>GPEKIRPECFELLRVLGKGGYGKVFQVRKVTGANTGKIFAMKVLKKAMIVRNAKDTAHTKAERNILEEVKHPFIVDLIYAFQTGGKLYLILEYLSGGELFMQLEREGIFMEDTACFYLAEISMALGHLHQKGIIYRDLKPENIMLNHQGHVKLTDFGLCKESIHDGTVTHTFCGTIEYMAPEILMRSGHNRAVDWWSLGALMYDMLTGAPPFTGENRKKTIDKILKCKLNLPPYLTQEARDLLKKLLKRNAASRLGAGPGDAGEVQAHPFFRHINWEELLARKVEPPFKPLLQSEEDV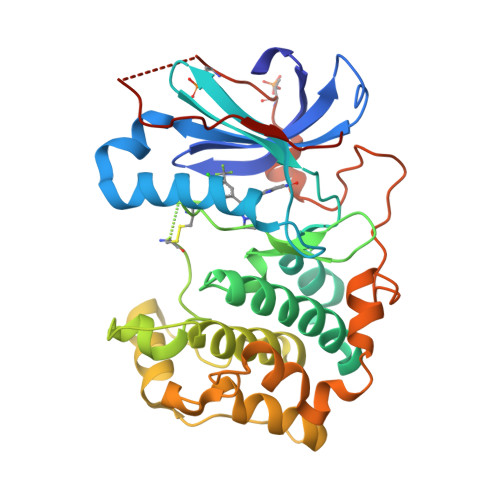SQFDSKFTRQTPVDSPDDSTLSESANQVFLGFEYVAPSVLES[2x]> GHMSGRGKKPTRTLVMTSMPSEKQNVVIQVVDKLKGFSIAPDVCETTTHVLSGKPLRTLNVLLGIARGCWVLSYDWVLWSLELGHWISEEPFELSHHFPAAPLCRSECHLSAGPYRGTLFADQPVMFVSPASSPPVAKLCELVHLCGGRVSQVPR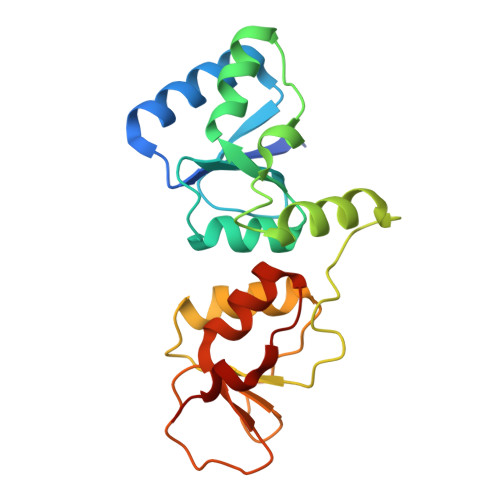QASIVIGPYSGKKKATVKYLSEKWVLDSITQHKVCAPENYLLSQ>MGHHHHHHHHHHSSGHIEGRHMPFPYSIDFVESKQNEQLLKDFHGERTGFVQVGEKRWFFPSRFKQYAESLYSFEARPDDTWIVTYPRSGTTWSQEMVWLLCNELDFETAKSIPLTQRFPFLEFHLFVHDEVKAEFLKENEHDVESMKFIEQLSQPAGFMLAEMKTPRFIKTHLPISLLPPSVFEQKAKIIYVARNPSDVAVSYYHLNRLYRTQGYVGDFETFYNYFEKDLTPWSPYWEHIKEGWAERDRENVLFMYYEDMKRNLPDTIRKTAAFLGKSFSDDQIDTMCTHLDIRNFRHNKSVTCEELKAVGILNSG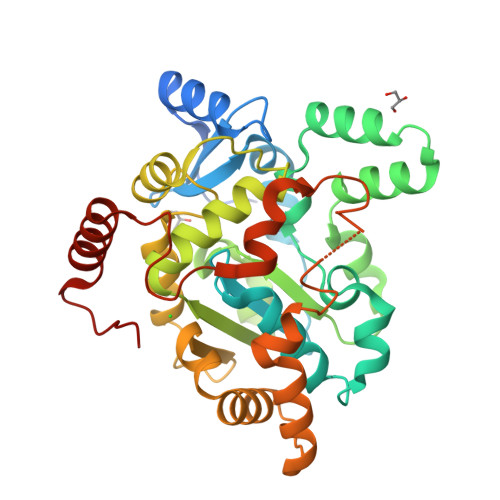EQGFVRNGQVRGNAEEMTDDIKRRLNEWTERNLNGTDIRFPDC[2x]> MNRMGGSVYANAMAQFAICRQPWNEYINLLTKQDSTPYHVEPQEKPAYRGRKRGREGWLFGQQVQLHYHRFPDEQLLTNLTRWRTGETVGDIALQQFRNAQPFDIEDKDPQGMQRPSPEVYMKLNYKNPATISRFLTRTGHMYPADILPLNPEAVAKLRVAKAQAVRIGLYPRFGNPFWFRSQKFRPKAYQENYDPTTYSTKHTMEHFAYNWVQTDRIRRYFKELEELQKNASNGARGGSATTAEQKQQNQFYAPE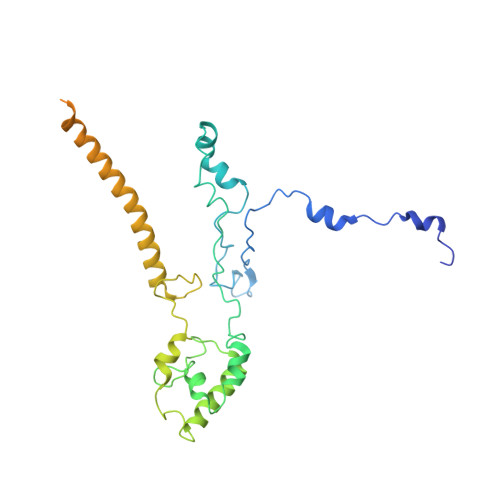NQPISMHRNNISYMAEVERSMKNPTVPGLMSTKGMKKKFHNLYSSTSTKRMGFSNPTLGIKKV> MVKNYDYKDDDDKGLSFFKRKKYSDKESLSSPETLEEKPNDELDPRVTEILERQIKADSYGASLVDLYGMLQGWEYCLAVAAYICSIVAGAALPLMTLIFGDMAQQFTDYSSGLHSNNQFVDKIDENALYFVYLGVGLLVFNYFATLLHIVVSEIIASRVREKFIWSILHQNMAYLDSLGSGEITSSITSDSQLIQQGVSEKIGLAAQSIATVVSALTVAFVIYWKLALVLLSVMVALILSSTPTILMLMQAYTDSIASYGKASSVAEEAFAAIKTATAFGAHEFQLQKYDEFILESKGYGKKKAISLALMMGSIWFIVFATYALAFWQGSRFMVSDNSGIGKILTACMAMLFGSLIIGNATISLKFVMVGLSAASKLFAMINREPYFDSASDAGEKINEFDGSISFRNVTTRYPSRPDITVLSDFTLDIKPGQTIALVGESGSGKSTVIALLERFYEYLDGEILLDGVDLKSLNIKWVRQQMALVQQEPVLFAASIYENVCYGLVGSKYENVTEKVKRELVEKACKDANAWEFISQMSNGLDTEVGERGLSLSGGQ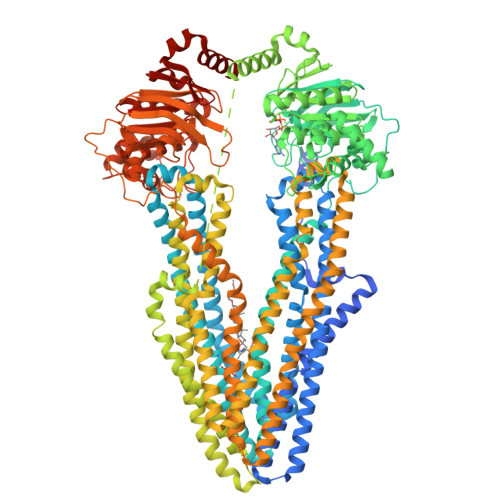KQRIAIARAVISEPKILLLDEATSALDTRSEGIVQDALNRLSETRTTIVIAHRLSTIQNADLIVVLSKGKIVETGSHKELLKKKGKYHQLVQIQNIRTKINNSGPQAPISLSNSSDLDSVSHKIDRVESLIYERAAADTIDESPVKKQSIPQLFLMLLQINKGDYYLLIPCLFLALIAGMGFPSFALLAGRVIEAFQVTGPQDFPHMRSLINKYTGFLFMIGCVLLIVYLFLTSFMVLSSESLVYKMRYRCFKQYLRQDMSFFDRPENKVGTLVTTLAKDPQDIEGLSGGTAAQLAVSVVIVVAGIILAVAVNWRLGLVCTATVPILLGCGFFSVYLLMVFEERILKDYQESASYACEQVSALKTVVSLTREVGIYEKYSNSIKDQVKRSARSVSRTTLLYALIQGMNPWVFALGFWYGSRLLLEGRATNREFFTVLMAILFGCQSAGEFFSYAPGMGKAKQAAINIRQVLDTRPKSIDIESEDGLKIDRLNLKGGIELRDVTFRYPTRPEVPVLTDLNLIIKPGQYVGLVGASGCGKSTTVGLIERFYDPESGQVLLDGVDIRDLHLRTYREVLALVQQEPVLFSGSIRDNIMVGSISDGADDGSEEDMIKACKDANIYDFISSLPEGFDTLCGNKGTMLSGGQKQRVAIARALIRNPRVLLLDEATSALDSESEMVVQDAIDKASKGRTTITIAHRLSTVQNCDVIYVFDAGRIVESGKHDELLQLRGKYYDLVQLQGLNAHHHHHHHHHH> GSHMASMILNSLSLCYHNKLILAPMVRVGTLPMRLLALDYGADIVYCEELIDLKMIQCKRVVNEVLSTVDFVAPDDRVVFRTC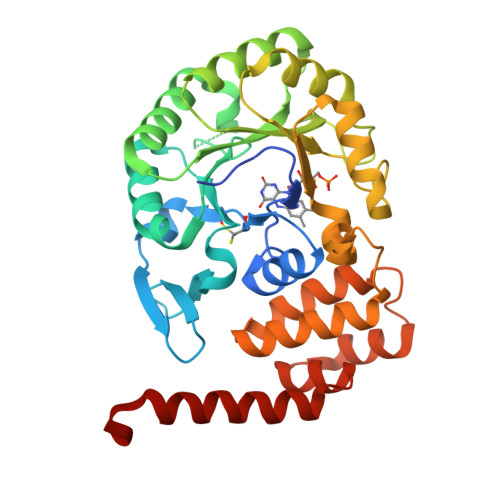EREQNRVVFQMGTSDAERALAVARLVENDVAGIDVNMGCPKQYSTKGGMGAALLSDPDKIEKILSTLVKGTRRPVTCKIRILPSLEDTLSLVKRIERTGIAAIAVHGRKREERPQHPVSCEVIKAIADTLSIPVIANGGSHDHIQQYSDIEDFRQATAASSVMVARAAMWNPSIFLKEGLRPLEEVMQKYIRYAVQYDNHYTNTKYCLCQMLREQLESPQGRLLHAAQSSREICEAFGLGAFYEETTQELDAQQARLSAKTSE> DLPRLIVYFQTTHDSSNRPISMLPLITEKGIALTHLIVCSFHINQGGVVHLNDFPPDDPHFYTLWNETITMKQAGVKVMGMVGGAAPGSFNTQTLDSPDSATFEHYYGQLRDAIVNFQLEGMDLDVEQPMSQQGIDRLI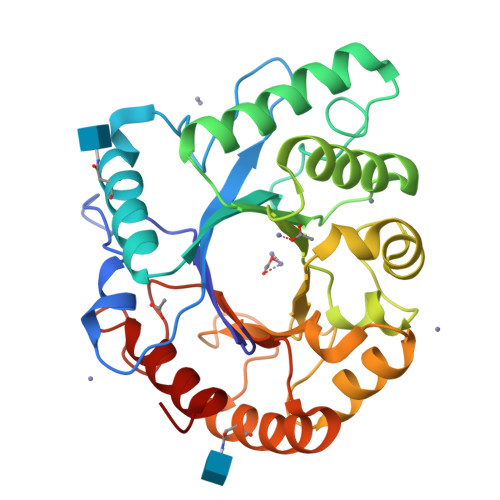ARLRADFGPDFLITLAPVASALEDSSNLSGFSYTALQQTQGNDIDWYNTQFYSGFGSMADTSDYDRIVANGFAPAKVVAGQLTTPEGAGWIPTSSLNNTIVSLVSEYGQIGGVMGWEYFNSLPGGTAEPWEWAQIVTVILRPGL3-(3,4-dihydroisoquinolin-2(1H)-ylsulfonyl)-N-methylbenzamide | 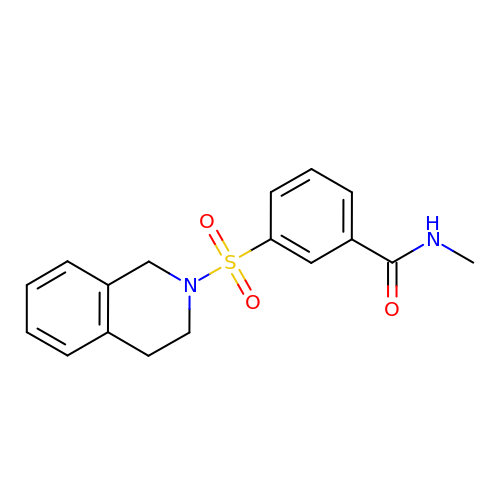C17 H18 N2 O3 S | PBBCJGRZQLBCCD-UHFFFAOYSA-N> QTSVSPSKVILPRGGSVLVTCSTSCDQPKLLGIETPLPKKELLLPGNNRKVYELSNVQEDSQPMCYSNCPD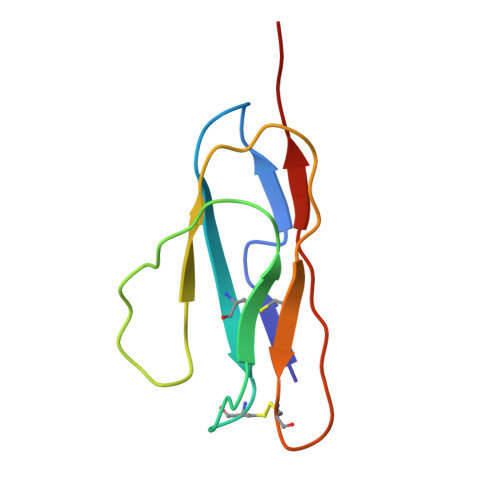GQSTAKTFLTVYWT2'-(beta-D-galactopyranosyloxy)-5-nitro[1,1'-biphenyl]-3-carboxylic acid | C19 H19 N 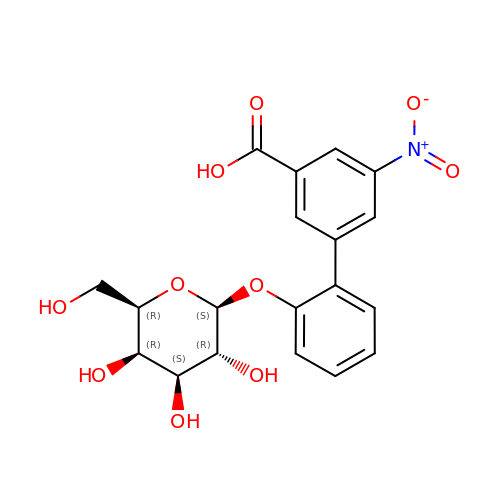O10 | GCARVRRYRBFOAI-DIKXUDHVSA-N> MNFIQYIDDSYAVKVKEINSSEGFYINGIQTPFFILSVFIGNKRVTGVEFNNYDSLPMLSVINDLGNIDLNVIPQNYFATAFTEIYFNIPF

In this study, we report a detailed characterization of ΦCjT23, an icosahedral temperate ssDNA phage with an inner lipid membrane, isolated earlier from a strain of Flavobacterium (previously Cytophaga). The virion structure determined by cryogenic electron microscopy reveals similarities to members of the viral kingdom Bamfordvirae that currently consists solely of dsDNA viruses with a major capsid protein composed of two upright β-sandwiches. The minimalistic structure of ΦCjT23 suggests that this phage serves as a model for the last common ancestor between ssDNA and dsDNA viruses in the Bamfordvirae. Both ΦCjT23 and the related phage FLiP infect Flavobacterium species found in several environments, suggesting that these types of viruses have a global distribution and a shared evolutionary origin.

Following the approach applied to the MCPs, we calculated a localized reconstruction of the internal part of ΦCjT23 spike (penton domain), in addition to the FLiP penton base from our previously published data. The resolutions of the localized reconstructions for ΦCjT23 and FLiP were 3.4 and 4.0 Å, respectively. In contrast to FLiP, the entire spike of ΦCjT23 is made by one protein, P13 (283 residues), which forms both the capsid-internal and capsid-external parts, analogously to the spike protein of phage PM212. The capsid-integral part of the spike, corresponding to the P13 N-terminal penton base domain (residues M1–F91), sits in a slightly raised position relative to the type 1 MCP trimers circling it. The penton base domain is a small β-barrel (SBB) with a β-strand topology that differs from the topologies of better-characterized SBBs29, and from the canonical β-sandwich fold observed in pentons of other viruses such as FLiP and Bamfordvirae members. The ΦCjT23 spike SBB is formed by anti-parallel β-strands β1, β2, and β4, and additional β-strands β3, β5, and β6. The region connecting strands β5 and β6 include a short α-helix (S55–D64) and a long loop (L65–F78). The α-helix resides at the monomer–monomer interface. Part of the loop (L65–N71) faces toward the central cavity of the pentamer. Together the five loops close an oculus in the middle of the pentamer.> MSGGFLRDDHLEFALHLHRRLAEAVPDGEVIWSPYSVACALGVLAAGARATTRTELTTLLGTDPAPLLAALDRAVTDSPDLASRTVLWVSADVPVRSSFRATMHDRPDSDVRTADFRTNPEGVRATVNADIADATRGMIRELLPQGAVTP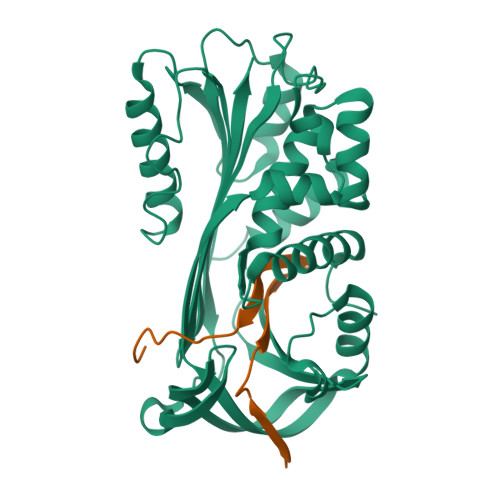DLRAILTNALWAKARWTTPFEAHLTREGTFRTPRGPKRVPFMHRTKTMPYATARGWRMVTLHAHDELAVDVLLPPGTNAAAVPTAPLLTALHRRSASTSVELALPRFELTQPHQLVEVLAEAGVRTLFTASADLSGISTVPLYVDTVIHQARLRVDERGAEGAAATAAMMLLA;> GAMPPRRTIRFSVDRPFHIVVRRRGAILFLGSIADPHDPGPAQ>[2x]MHHHHHHSSGRENLYFQGPEQPFIVLGQEEYGEHHSSIMHCRVDCSGRRVASLDVDGVIKVWSFNPIMQTKASSISKSPLLSLEWATKRDRLLLLGSGVGTVRLYDTEAKKNLCEININDNMPRILSLACSPNGASFVCSAAAPSLTSQVDFSAPDIGSKGMNQVPGRLLLWDTKTMKQQLQFSLDPEPIAINCTAFNHNGNLLVTGAADGVIRLFDM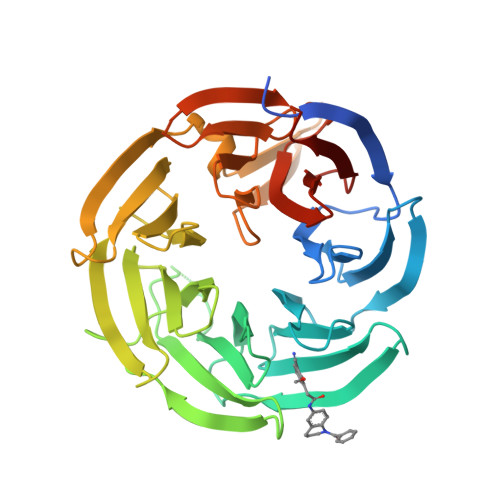QQHECAMSWRAHYGEVYSVEFSYDENTVYSIGEDGKFIQWNIHKSGLKVSEYSLPSDATGPFVLSGYSGYKQVQVPRGRLFAFDSEGNYMLTCSATGGVIYKLGGDEKVLESCLSLGGHRAPVVTVDWSTAMDCGTCLTASMDGKIKLTTLLAHKA>[2x]AECSVDIQGNDQMQFNTNAITVDKS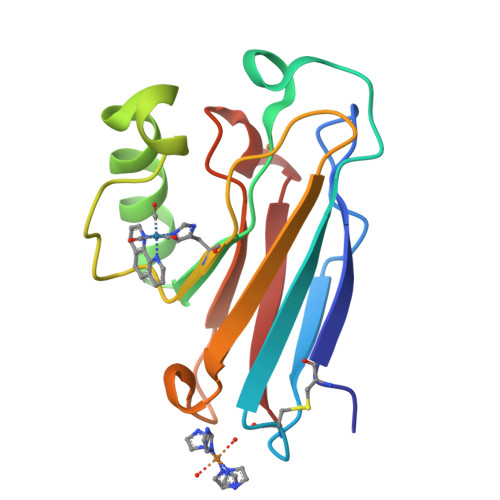CKQFTVNLSHPGNLPKNVMGHNWVLSTAADMQGVVTDGMASGLDKDYLKPDDSRVIAHTKLIGSGEKDSVTFDVSKLKEGEQYMFFCTFPGHSALMKGTLTLK> GSGTTYIFSKGGGQITYKWPPNDRPS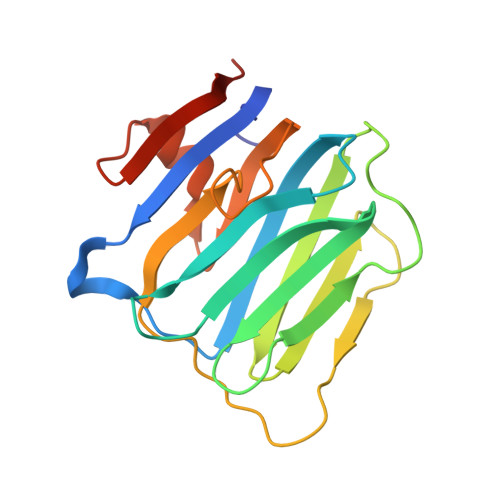TRADRLAIGFSTVQKEAVLVRVDSSSGLGDYLELHIHQGKIGVKFNVGTDDIAIEESNAIINDGKYHVVRFTRSGGNATLQVDSWPVIERYPAGRQLTIFNSQATIIIGGKEQGQPFQGQLSGLYYNGLKVLNMAAENDANIAIVGNVRLVGEVS> MRKELVFVLLALFL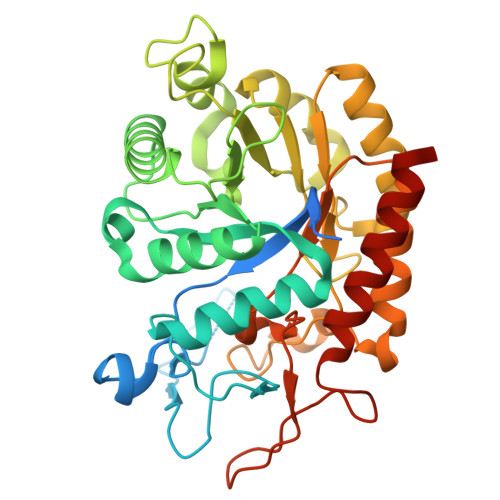CAGCNGNKKKMNGEHDLDAANITLDDHTISFYYNWYGNPSVDGEMKHWMHPIALAPGHSGLVGAISGLNDDIACNFYPELGTYSSNDPEIIRKHIRMHIKANVGVLSVTWWGESDYGNQSVSLLLDEAAKVGAKVCFHIEPFNGRSPQTVRENIQYIVDTYGDHPAFYRTHGKPLFFIYDSYLIKPAEWAKLFAAGGEISVRNTKYDGLFIGLTLKESELPDIETACMDGFYTYFAATGFTNASTPANWKSMQQWAKAHNKLFIPSVGPGYIDTRIRPWNGSTTRDRENGKYYDDMYKAAIESGASYISITSFNEWHEGTQIEPAVSKKCDAFEYLDYKPLADDYYLIRTAYWVDEFRKARSASEDVQ>MDTSMKEKVKAKLVEIRKFVPFIRRVRIDFQDTLSKV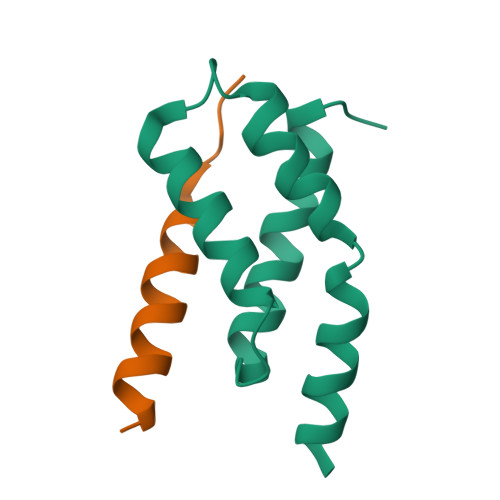QGHRLDALVNLLDREDVSMSSLNKIEVIIDKLRTRFNPRIE[4x];>[4x]SMEPKIKEDADNAMLDSLLADPFENNSP>TYKKPSDAELKRTLTEEQYQVTQNSATEYAFSHEYDHLFKPGI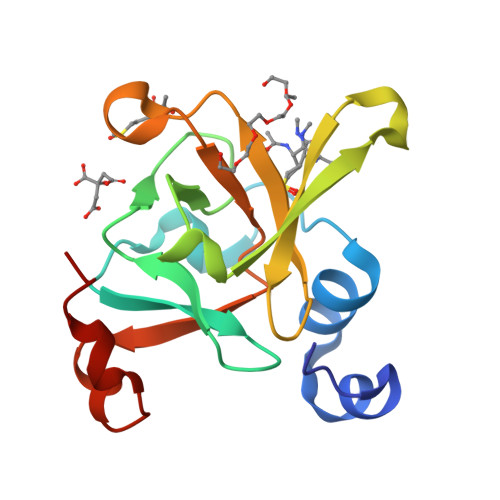YVDVVSGEPLFSSADKYDSGSGWPSFTRPIDAKSVTEHDDFSYNMRRTEVRSHAADSHLGHVFPDGPRDKGGLRYSINGASLKFIPLEQMDAAGYGALKSKVK[2x]8-nitro-3,7-dihydro-1H-purine-2,6-dione | C5 H3 N5 O4 | 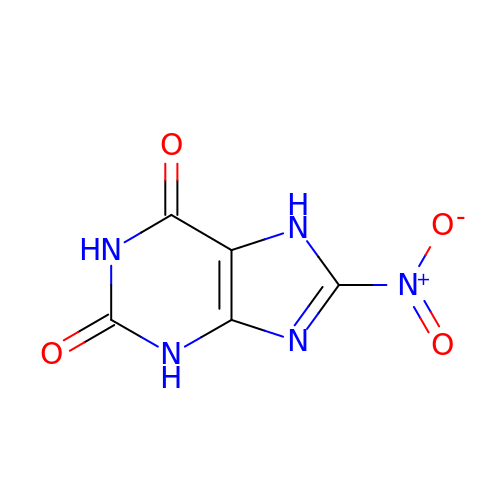LXDVSSPKQAHSGS-UHFFFAOYSA-N> ADPPPVHDTDGHELRADANYYVLSANRAHGGGLTMAPGHGRHCPLFVSQDPNGQHDGFPVRITPYGVAPSDKIIRLSTDVRISFRAYTTCLQSTEWHIDSELAAGRRHVITGPVKDPSPSGRENAFRIEKYSGAEVHEYKLMSCGDWC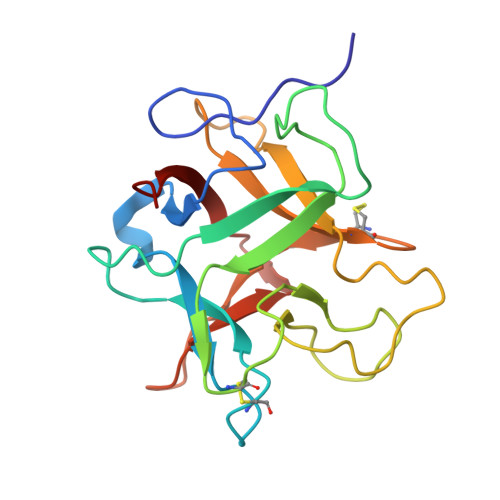QDLGVFRDLKGGAWFLGATEPYHVVVFKKAPPA> MSGYDRALSIFS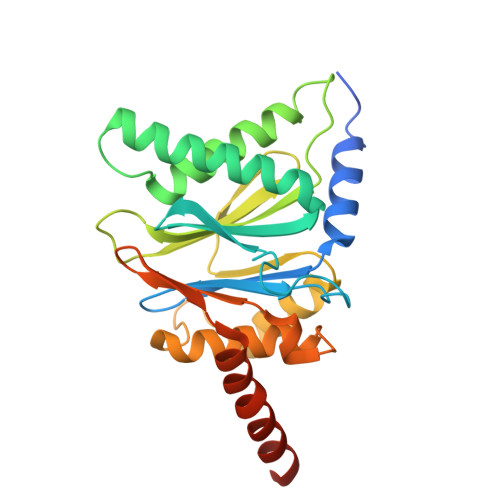PDGHIFQVEYALEAVKRGTCAVGVKGKNCVVLGCERRSTLKLQDTRITPSKVSKIDSHVVLSFSGLNADSRILIEKARVEAQSHRLTLEDPVTVEYLTRYVAGVQQRYTQSGGVRPFGVSTLIAGFDPRDDEPKLYQTEPSGIYSSWSAQTIGRNSKTVREFLEKNYDRKEPPATVEECVKLTVRSLLEVVQTGAKNIEITVVKPDSDIVALSSEEINQYVTQIEQEKQEQQEQDKKKKSNH>SKFLDRFRYFKQKGETFADGHGQLLNTNRDWEDGYRQRWQHDKIVRSTHGVNCTGSCSWKIYVKNGLVTWETQQTDYPRTRPDLPNHEPRGCPRGASYSWYLYSANRLKYPMMRKRLMKMWREAKALHSDPVEAWASIIEDADKAKSFKQARGRGGFVRSSWQEVNELIAASNVYTIKNYGPDRVAGFSPIPAMSMVSYASGARYLSLIGGTCLSFYDWYCDLPPASPQTWGEQTDVPESADWYNSSYIIAWGSNVPQTRTPDAHFFTEVRYKGTKTVAVTPDYAEIAKLCDLWLAPKQGTDAAMALAMGHVMLREFHLDNPSQYFTDYVRRYTDMPMLVMLEERDGYYAAGRMLRAADLVDALGQENNPEWKTVAFNTNGEMVAPNGSIGFRWGEKGKWNLEQRDGKTGEETELQLSLLGSQDEIAEVGFPYFGGDGTEHFNKVELENVLLHKLPVKRLQLADGSTALVTTVYDLTLANYGLERGLNDVNCATSYDDVKAYTPAWAEQITGVSRSQIIRIAREFADNADKTHGRSMIIVGAGLNHWYHLDMNYRGLINMLIFCGCVGQSGGGWAHYVGQEKLRPQTGWQPLAFALDWQRPARHMNSTSYFYNHSSQWRYETVTAEELLSPMADKSRYTGHLIDFNVRAERMGWLPSAPQLGTNPLTIAGEAEKAGMNPVDYTVKSLKEGSIRFAAEQPENGKNHPRNLFIWRSNLLGSSGKGHEFMLKYLLGTEHGIQGKDLGQQGGVKPEEVDWQDNGLEGKLDLVVTLDFRLSSTCLYSDIILPTATWYEKDDMNTSDMHPFIHPLSAAVDPAWEAKSDWEIYKAIAKKFSEVCVGHLGKETDIVTLPIQHDSAAELAQPLDVKDWKKGECDLIPGKTAPHIMVVERDYPATYERFTSIGPLMEKIGNGGKGIAWNTQSEMDLLRKLNYTKAEGPAKGQPMLNTAIDAAEMILTLAPETNGQVAVKAWAALSEFTGRDHTHLALNKEDEKIRFRDIQAQPRKIISSPTWSGLEDEHVSYNAGYTNVHELIPWRTLSGRQQLYQDHQWMRDFGESLLVYRPPIDTRSVKEVIGQKSNGNQEKALNFLTPHQKWGIHSTYSDNLLMLTLGRGGPVVWLSEADAKDLGIADNDWIEVFNSNGALTARAVVSQRVPAGMTMMYHAQERIVNLPGSEITQQRGGIHNSVTRITPKPTHMIGGYAHLAYGFNYYGTVGSNRDEFVVVRKMKNIDWLDGEGNDQVQESVK[2x];>MKIRSQVGMVLNLDKCIGCHTCSVTCKNVWTSREGVEYAWFNNVETKPGQGFPTDWENQEKYKGGWIRKINGKLQPRMGNRAMLLGKIFANPHLPGIDDYYEPFDFDYQNLHTAPEGSKSQPIARPRSLITGERMAKIEKGPNWEDDLGGEFDKLAKDKNFDNIQKAMYSQFENTFMMYLPRLCEHCLNPACVATCPSGAIYKREEDGIVLIDQDKCRGWRMCITGCPYKKIYFNWKSGKSEKCIFCYPRIEAGQPTVCSETCVGRIRYLGVLLYDADAIERAASTENEKDLYQRQLDVFLDPNDPKVIEQAIKDGIPLSVIEAAQQSPVYKMAMEWKLALPLHPEYRTLPMVWYVPPLSPIQSAADAGELGSNGI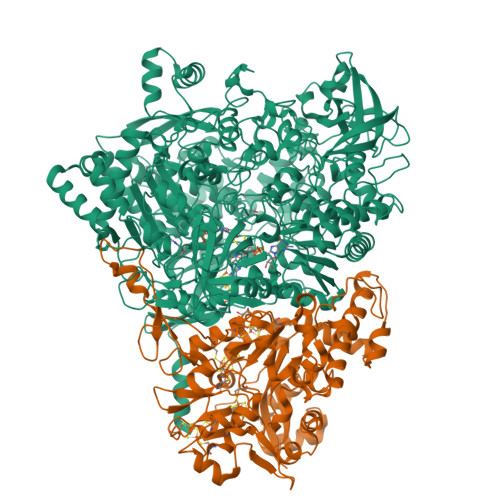LPDVESLRIPVQYLANLLTAGDTKPVLRALKRMLAMRHYKRAETVDGKVDTRALEEVGLTEAQAQEMYRYLAIANYEDRFVVPSSHRELAREAFPEKNGCGFTFGDGCHGSDTKFNLFNSRRIDAIDVTSKTEPHP[2x]> MTAAPASPQQMRDRLLQAIDSQ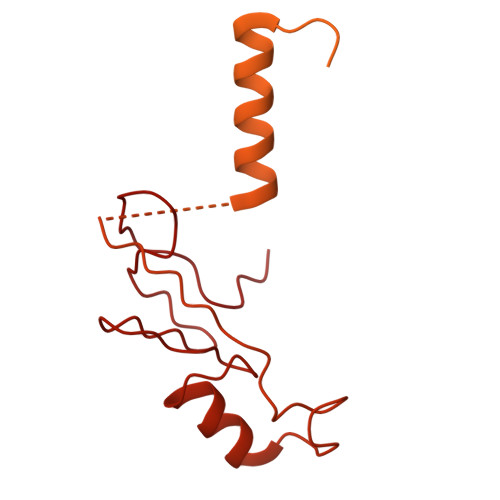SNIRNMVAVLEVISSLERYPITKEALEETRLGKLINDVRKKTKNEELAKRAKRLLRSWQKLIEPVHQNEVALRALAGAAGSANGGAHNCRPEMGVAGAPKSIHDLKNRNDIQRLPGQRLDRLGSRKRRGDQRDLGHPGPPHKVSKGSPDPLVPNASPLPTNGISGSPESLPSPLDGSGHLGPDGSRLEPSDNEKHSTKIPVNAVRPRPSSPGLGKPPVPCLQTKAAQLQQLDRADESPGPPYPRGSSRCSFSPRNSRHEGSFSRHRSSYIPKGQVSSPSPWPQPPDNTQVPSPLPLAQPPTPPVRRQELLPNAESPVHWPEQSEGHPRLTGPACRAGFSPDSSKADSDATSSGGSDSKKKKRYRPRDYTVNLDGQVAEAGVKPVRLKERKLTFDPMTRQIRPLTQKEPVRADSPVPTEQLPRTELEQQEVKASLQSPFEQTNWKELSRNEIIQSYLSRQSSLLSSSGAQTPGAHHFMAEYLKQEESSRQGARQPHVLLPLPTPTDLPGLTREVTQDDLDRIQAQQWPGVNGCEDTQGNWYDWTQCISLDPHGDDGRLNILPYVCLD>[2x]MGNIMSASFAPECTDLKTKYDSCFNEWYSEKFL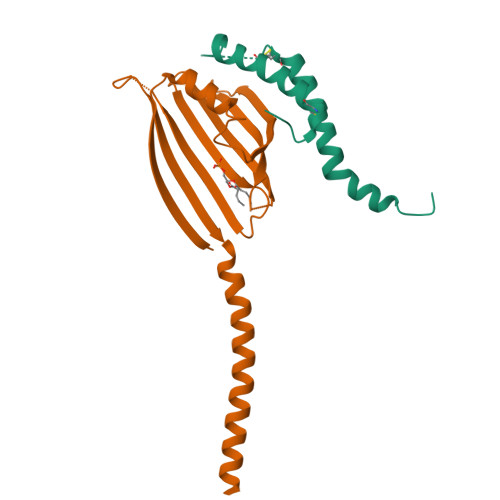KGKSVENECSKQWYAYTTCVNAALVKQGIKPALDEAREEAPFENGGKLKEVDK;>[2x]MGSSHHHHHHSQDPMVLLHKSTHIFPTDFASVSRAFFNRYPNPYSPHVLSIDTISRNVDQEGNLRTTRLLKKSGKLPTWVKPFLRGITETWIIEVSVVNPANSTMKTYTRNLDHTGIMKVEEYTTYQFDSATSSTIADSRVKFSSGFNMGIKSKVEDWSRTKFDENVKKSRMGMAFVIQKLEEARNPQF[(2~{S},4~{R},5~{R})-5-(6-aminopurin-9-yl)-4-oxidanyl-oxolan-2-yl]methyl phosphono hydrogen phosphate | C10 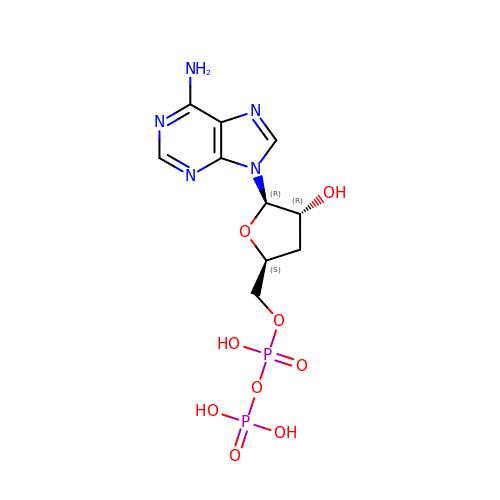H15 N5 O9 P2 | OBEBFUHFXYDSAW-BAJZRUMYSA-N>[3x]NVEEETKYIELMIVNDHLMFKKHRLSVVHTNTYAKSVVNMADLIYKDQLKTRIVLVAMETWATDNKFAISENPLITLREFMKYRRDFIKEKSDAVHLFSGSQFESSRSGAAYIGGICSLLKGGGVNEFGKTDLMAVTLAQSLAHNIGIISDKRKLASGECKCEDTWSGCIMGDTGYYLPKKFTQCNIEEYHDFLNSGGGACLFNKPSKLLDPPECGNGFIETGEECDCGTPAECVLEGAECCKKCTLTQDSQCSDGLCCKKCKFQPMGTVCREAVNDCDIRETCSGNSSQCAPNIHKMDGYSCDGVQGICFGGRCKTRDRQCKYIWGQKVTASDKYCYEKLNIEGTEKGNCGKDKDTWIQCNKRDVLCGYLLCTNIGNIPRLGELDGEITSTLVVQQGRTLNCSGGHVKLEEDVDLGYVEDGTPCGPQMMCLEHRCLPVASFNFSTCLSSKEGTICSGNGVCSNELKCVCNRHWIGSDCNTYFPHNDDAKTGITLSG;>[3x]DAAQPARRARRTYEAYPAKPKCPAVCTCTKDNALCENARSIPRTVPPDVISLSFVRSGFTEISEGSFLFTPSLQLLLFTSNSFDVISDDAFIGLPHLEYLFIENNNIKSISRHTFRGLKSLIHLSLANNNLQTLPKDIFKGLDSLTNVDLRGNSFNCDCKLKWLVEWLGHTNATVEDIYCEGPPEYKKRKINSLSSKDFDCIITEFAKSQDLPYQSLSIDTFSYLNDEYVVIAQPFTGKCIFLEWDHVEKTFRNYDNITGTSTVVCKPIVIETQLYVIVAQLFGGSHIYKRDSFANKFIKIQDIEILKIRKPNDIETFKIENNWYFVVADSSKAGFTTIYKWNGNGFYSHQSLHAWYRDTDVEYLEIVRTPQTLRTPHLILSSSSQRPVIYQWNKATQLFTNQTDIPNMEDVYAVKHFSVKGDVYICLTRFIGDSKVMKWGGSSFQDIQAMPSRGSMVFQPLQINNYQYAILGSDYSFTQVYNWDAEKAKFVKFQELNVQAPRSFTHVSINKRNFLFASSFKGNTQIYKHVIVDLSAKHHHHHH

LGI1 is a 60 kDa secreted neuronal protein that consists of the N-terminal leucine-rich repeat (LRR) domain and the C-terminal epitempin-repeat (EPTP) domain (Staub et al., 2002). Meanwhile, the S473L mutation of LGI1 causes epileptiform seizures due to reduced binding to ADAM22, which is a member of the A disintegrin and metalloproteinase (ADAM) family and acts as a receptor for LGI1 in neurons without protease activity. The ectodomain (ECD) of ADAM22 consists of a metalloprotease-like domain, a disintegrin domain, a cysteine-rich domain, and an EGF-like domain (Liu et al., 2009). As such, the LGI1–ADAM22 complex maintains normal nerve signal transduction through the interaction network, including synaptic ion channels.

In this study, the 3D structure of the 3:3 LGI1–ADAM22ECD complex was determined at a nominal resolution of 3.79 Å by cryo-EM single-particle analysis. LGI1EPTP interacts with the metalloprotease-like domain of ADAM22 to form the LGI1EPTP–ADAM22ECD complex, while the LRR domain of one LGI1 molecule interacts with the EPTP domain of the neighboring LGI1, thereby bridging three distant ADAM22 molecules in the 3:3 complex. Like the crystal structure of the 2:2 LGI1–ADAM22ECD complex, the LRR and EPTP domains of LGI1 are linked by a two-residue linker (Ile222–Ile223) in an extended conformation. When the three assembled LGI1–ADAM22ECD complexes were superposed with the LGI1EPTP–ADAM22ECD structure as the reference, all three LGI1 LRR domains were oriented differently. Although the triangular shape observed in the 2D class-averaged image suggested (pseudo-)C3 symmetry of the 3:3 complex, the determined structure of the 3:3 complex was not symmetric. We then analyzed the interdomain motion of the three LGI1 domains (assigned to chains B, D, and F in the deposited PDB file) in the 3:3 LGI1–ADAM22ECD complex by the DynDom server (Veevers and Hayward, 2019). The LRR domain of chain D was rotated 69.8° around the hinge axis compared to chain B, and the LRR domain of chain F was rotated 69.0° around the hinge axis compared to chain B. The LRR domains of chain D and chain F were also rotated 70.0° around the hinge axis relative to each other, suggesting that each LRR domain rotates approximately 70° about the hinge axis in the 3:3 LGI1–ADAM22ECD complex. On the other hand, the density of the disintegrin, cysteine-rich, and EGF-like domains after Pro445 of ADAM22 is relatively weak in all three molecules. Using three orthogonal principal modes, the 3D VA indicated two twisting motions and one stretching motion of the triangular-shaped 3:3 LGI1–ADAM22ECD complex (Animation 3–5). This analysis also visualized relatively large motions of the disintegrin, cysteine-rich, and EGF-like domains of ADAM22 (Animation 3–5), suggestive of intrinsic conformational flexibilities of these domains, likely resulting in lower local resolution in the periphery of the complex.>MGACPPKAKGPWAQLQKLLISWPVGEQDWEQYRDRVNMLQQERIRDSPLLQAAKENDLRLLKILLLNQSCDFQQRGAVGETALHVAALYDNLEAATLLMEAAPELAKEPALCEPFVGQTALHIAVMNQNLNLVRALLARGASVSARATGAAFRRSPHNLIYYGEHPLSFAACVGSEEIVRLLIEHGADIRAQDSLGNTVLHILILQPNKTFACQMYNLLLSYDEHSDHLQSLELVPNHQGLTPFKLAGVEGNTVMFQHLMQKRKHVQWTCGPLTSTLYDLTEIDSWGEELSFLELVVSSKKREARQILEQTPVKELVSFKWKKYGRPYFCVLASLYILYMICFTTCCIYRPLKLRDDNRTDPRDITILQQKLLQEAYVTHQDNIRLVGELVTVTGAVIILLLEIPDIFRVGASRYFGQTILGGPFHVIIITYASLVLLTMVMRLTNMNGEVVPLSFALVLGWCSVMYFARGFQMLGPFTIMIQKMIFGDLMRFCWLMAVVILGFASAFHITFQTEDPNNLGEFSDYPTALFSTFELFLTIIDGPANYSVDLPFMYCITYAAFAIIATLLMLNLFIAMMGDTHWRV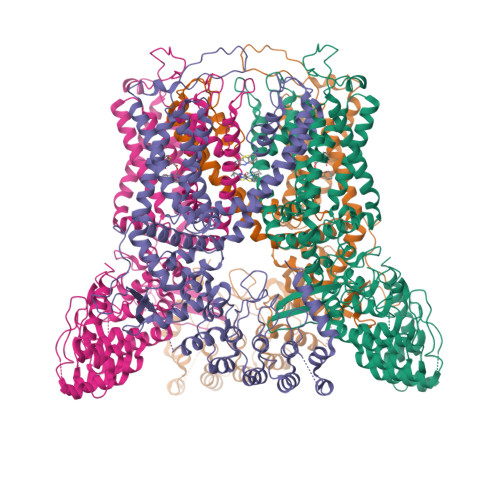AQERDELWRAQVVATTVMLERKMPRFLWPRSGICGYEYGLGDRWFLRVENHHDQNPLRVLRYVEAFKCSDKEDGQEQLSEKRPSTVESGMLSRASVAFQTPSLSRTTSQSSNSHRGWEILRRNTLGHLNLGLDLGEGDGEEVYHF[4x]[(2S)-2-octadecanoyloxypropyl] octadecanoate 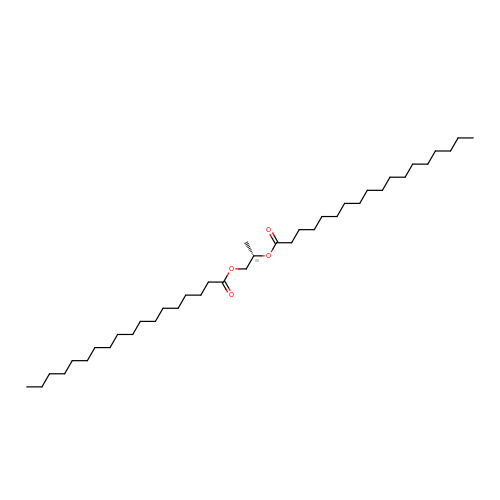| C39 H76 O4 | JEMDXOYRWHZUCG-QNGWXLTQSA-N>SLDRADILYNIRQTSRPDVIPTQRDRPVAVSVSLKFINILEVNEITNEVDVVFWQQTTWSDRTLAWDSSHSPDQVSVPISSLWVPDLAAYNAISKPEVLTPQLARVVSDGEVLYMPSIRQRFSCDVSGVDTESGATCRIKIGSWTHHSREISVDPTTENSDDSEYFSQYSRFEILDVTQKK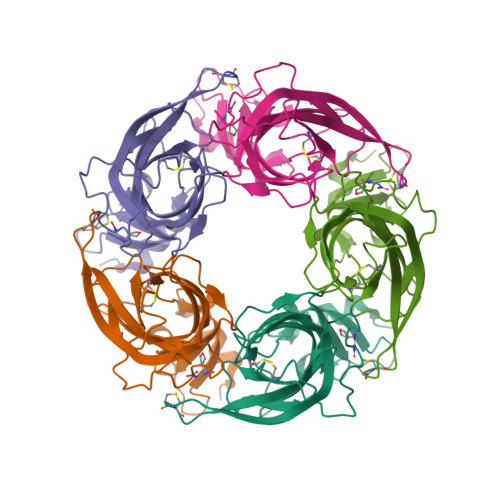NSVTYSCCPEAYEDVEVSLNFRKKGRSE[5x]Contractile bacteriophages of the family Myoviridae (i.e. T4), R-type pyocins and the type VI secretion system (T6SS) of Gram-negative bacteria are evolutionarily related nano-scale injection machines that puncture target cell membranes using a shared contraction mechanism. TssA subunits are enigmatic as they possess a conserved N-terminal region of unknown function, previously identified as ImpA_N (PFAM: PF0681226), whereas sequences located C-terminal to this region are highly divergent. Consistent with this, phylogenetic analysis has suggested that the TssA family can be subdivided into three clades (TssA1, TssA2 and TssA3). The structural studies presented here show that TssA1B, TssA2A and TssA2B possess structurally diverse CTDs that lead to distinct overall architectures for their respective complexes.

The structure of an Ah TssA2A Nt2 domain construct (D231-L374) was solved to 1.76 Å with four subunits (chains A–D) in the asymmetric unit arranged as two independent dimers, consistent with previous SEC analysis, that showed that Ah TssA2A Nt2 exists as dimers in solution. Each monomer folds into a cluster of seven α-helices (α1–α7), the arrangement of which is very similar to that of the EAEC TssA2B Nt2 domain (RMSD = 2.0 Å) as determined by structural alignment. Specifically, the related regions include helices α1-α5 of Bc TssA1B Sd1 (i.e. most of the ImpA_N region) and α2–α6 of Ah TssA2A Nt2. This similarity suggests that an ancient gene duplication event may have played a role in the evolution of the Nt1 and Nt2 domains of TssA2 subunits. Following refinement, these dimers could be seen to be essentially identical in structure to that of the dimer formed by the isolated TssA2A Nt2 domain (RMSD = 0.4 Å).

>MSYQHPWCARLLTSLPDEQIRGAVLADEPRWDYVETELVKLGSLAHSQVDLNAVAEACLGLLESRTKDMRVLAQLLRCLQHPAKATPLGAAISLLEAWIQAYWLLAWPGNASQKQRLMVQIVKRFEGALPRICESASAAELAQLLAQAEQLERVWLAQCPDKGELLDPLVMGLKRAQRQQLAQAEANAAGQPQSSGAAAAGSPASVASTASCAGAMVLSGSAGVDVDSSNDRAWRQTQLKVAELLIERQPEVAVGYRLRRHAVWAGITAVPMSGAGNKTPLAPMSADMVDEYRAAMNAPDQGLWQRIEQSLTLAPYWFEGHRLSAEVAEKLGFGAVAQAIAEELGTFLQRLPALRELAFSDGSPFLSPECSRWLLEHHHHHH[4x]> IESIIKTATDTVKSEINAELG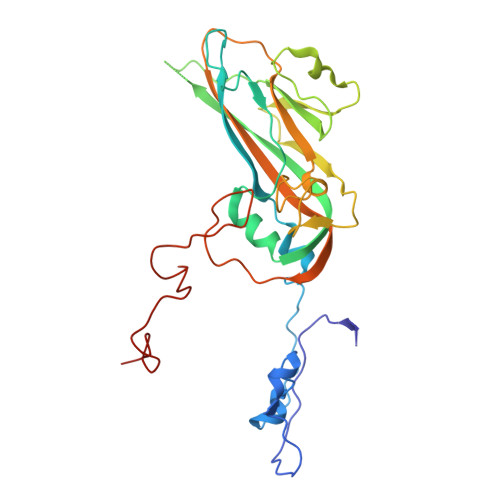VVPSLNAVETGATSNTEPEEAIQTRTVINQHGVSETLVENFLSRAALVSKRSFEYKDHTSSAAQTDKNFFKWTINTRSFVQLRRKLELFTYLRFDAEITILTTVAVNGSSNNTYMGLPNLTLQAMFVPTGALTPEKQDSFHWQSGSNASVFFKISDPPARMTIPFMCINSAYSVFYDGFAGFEKSGLYGINPADTIGNLCVRIVNEHQPVGFTVTVRVYMKPKHIKAWAPRPPRTLPYMSIANANYKGKKRAPNALNAIIGNRDSVKTMPHNIVTT> MGNCHTVGPNEALVVSGGCCGSDYKQYVFGGWAWAWWCISDTQRLSLEVMTILCRCENIETSEGVPLFVTGVAQVKIMTEKELLAVACEQFLGKNVQDIKNVVLQTLEGHLRSILGTLTVEQIYQDRDQFAKLVREVAAPDVGRMGIEILSFTIKDVYDKVDYLSSLGKTQTAVVQRDADIGVAEAERDAGIREAECKKEMLDVKFMADTKIADSKRAFELQKSAFSEEVNIKTAEAQLAYELQGAREQQKIRQEEIEIEVVQRKKQIAVEA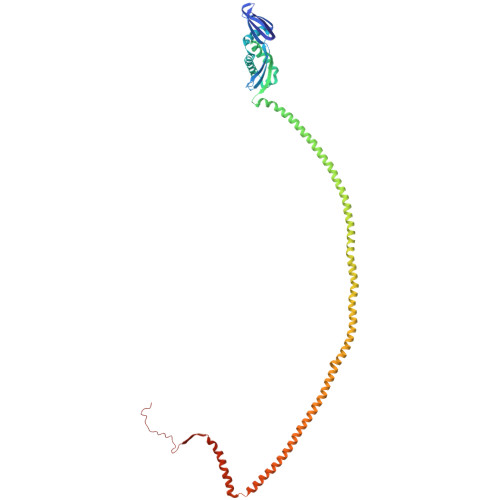QEILRTDKELIATVRRPAEAEAHRIQQIAEGEKVKQVLLAQAEAEKIRKIGEAEAAVIEAMGKAEAERMKLKAEAYQKYGDAAKMALVLEALPQIAAKIAAPLTKVDEIVVLSGDNSKVTSEVNRLLAEL> NEVTLLDSRSVQGELGWIASPLEGGWEEVSIMDEKNTPIRTYQVCNVMEPSQNNWLRTDWITREGAQRVYIEIKFTLRDCNSLPGVMGTCKETFNLYYYESDNDKERFIRENQFVKIDTIAADESFTQVDIGDRIMKLNTEIRD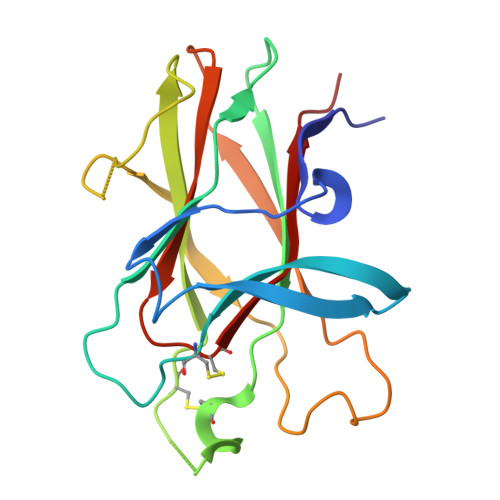VGPLSKKGFYLAFQDVGACIALVSVRVFYKK> MTENILRKSDEEIQKEITARVKALESMLIEQGILTTSMIDRMAEIYENEVGPHLGAKVVVKAWTDPEFKKRLLADGTEACKELGIGGLQGEDMMWVENTDEVHHVVVCTL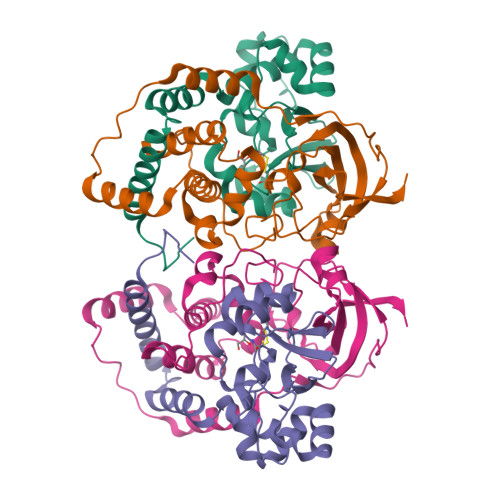CACYPWPVLGLPPNWFKEPQYRSRVVREPRQLLKEEFGFEVPPSKEIKVWDSSSEMRFVVLPQRPAGTDGWSEEELATLVTRESMIGVEPAKAV;> MNGVYDVGGTDGLGPINRPADEPVFRAEWEKVAFAMFPATFRAGFMGLDEFRFGIEQMNPAEYLESPYYWHWIRTYIHHGVRTGKIDLEELERRTQYYRENPDAPLPEHEQKPELIEFVNQAVYGGLPASREVDRPPKFKEGDVVRFSTASPKGHARRARYVRGKTGTVVKHHGAYIYPDTAGNGLGECPEHLYTVRFTAQELWGPEGDPNSSVYYDCWEPYIELVDT> MSPLSGSLAPLNMKGLVKFQDVSFAYPNHPNVQVLQGLTFTLYPGKVTALVGPNGSGKSTVAALLQNLYQPTGGKVLLDGEPLVQYDHHYLHTQVAAVGQEPLLFGRSFRENIAYGLTRTPTMEEITAVAMESGAHDFISGFPQGYDTEVGETGNQLAVGQRQAVALARALIRKPRLLILDNATSALDAGNQLRVQRLLYESPEWASRTVLLITQQLSLAERAHHILFLKEGS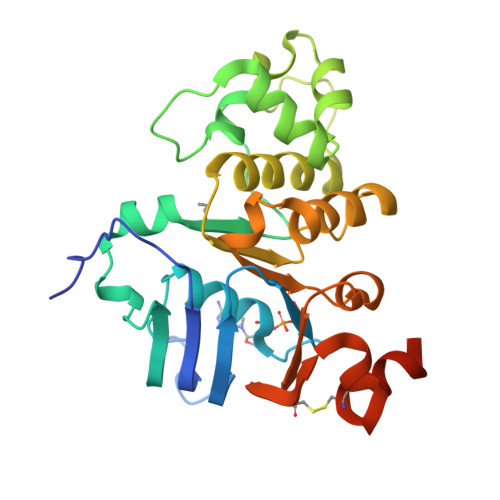VCEQGTHLQLMERGGCYRSMVEALAAPSDAAAHHHHHH>[6x]GASGDLYEVERIVDKRKNKKGKWEYLIRWKGYGSTEDTWE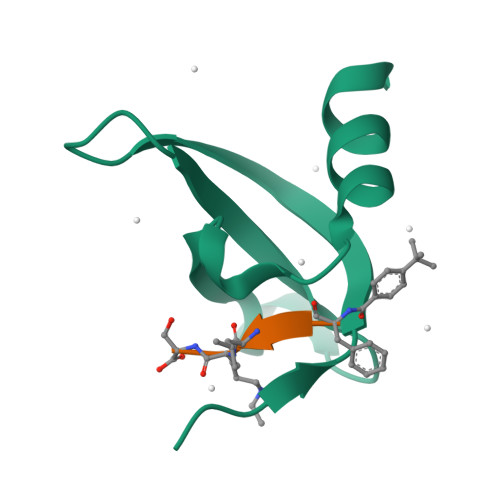PEHHLLHCEEFIDEFNGLHMSKDK While chemical methylation of an amide bond uses a strong base to generate the imidate, OphA, the precursor protein of the fungal peptide macrocycle omphalotin A, self-hypermethylates amides at pH 7 using S-adenosyl methionine (SAM) as cofactor. Omphalotin A derives from the C terminus of the OphA protein, and it is the OphA protein that methylates its own C terminus using S-adenosyl methionine (SAM). The structure of OphA reveals a complex catenane-like arrangement in which the peptide substrate is clamped with its amide nitrogen aligned for nucleophilic attack on the methyl group of SAM. Here, we report the structure of the peptide amide methyltransferase OphA including complexes with cofactor [SAM and S-adenosyl homocysteine (SAH)], cofactor analog, substrate, and product.

Superposition of both sinefungin complexes with the OphAΔC6 Y63F-SAH, OphAΔC18-SAM, and OphAΔC18-SAH complexes shows similar consistency in the protein structure, cofactor, and where present substrate positions. We conclude that the extensive hydrogen-bonding network at the active site and the catenane-like arrangement lead to a highly rigid active site. In both sinefungin complexes, the two nitrogen atoms (sinefungin and amide) approach close enough to form a hydrogen bond (distance varies between 3.1 and 3.3 Å).

> GTSTQTKAGSLTIVGTGIESIGQMTLQALSYIEAAAKVFYCVIDPATEAFILTKNKNCVDLFQYYDNGKSRLNTYTQMSELMVREVRKGLDVVGVFYGHPGVFVNPSHRALAIAKSEGYRARMLPGVSAEDCLFADLCIDPSNPGCLTYEASDFLIRDRPVSIHSHLVLFQVGCVGIADFNFTGFDNNKFGVLVDRLEQEYGAEHPVVHYIAAMMPHQDPVTDKYTVAQLREPEIAKRVGGVSTFYIPPKARKASNLDIIRRLELLPAGQVPDKKARIYPANQWEPDVPEVEPYRPSDQAAIAQLADHAPPEQYQPLATSKAMSDVMTKLALDPKALADYKADHRAFAQSVPDLTPQERAALELGDSWAIRCAMKNMPSSLLDAARESGEEASQNGFPWVIVVGVIGVIG>[2x]AEAESALEYAQQALEKAQLALQAARQALKA

In this work, we demonstrate the first ever high-resolution structure of co-assembly between a protein and buckminsterfullerene (C60), which suggests a simple structural mode for protein–fullerene co-organization. As in the protein-only structure, COP forms a canonical tetrameric anti-parallel coiled coil. Each tetramer presents four tyrosine residues (one per monomer) in exterior c positions of the coiled-coil heptad, and each of these engages a C60 moiety. One C60 is wedged between two Tyr residues donated by adjacent tetramers, such that two tetramers are needed to coordinate one C60.

Crystals from the resulting suspension grew within 24 h in several conditions, and three separate structures of the C60Sol–COP complex were resolved to 1.67, 1.76 and 2.35 Å, respectively. Furthermore, the three different COP–C60Sol co-crystals obtained under different conditions all produced effectively identical binding interfaces and assembly geometries, arguing that fullerene may have a strong preference for the observed coordination geometry. The interaction between COP and the fullerene group involves non-polar contacts, with C60 fitting perfectly into a symmetric hydrophobic cavity created by helices of two adjacent COP tetramers. The dominant contact appears to be the π–π aromatic stacking between C60 and Tyr9, donated by each tetramer, while several aliphatic carbons line the pocket to further support the bound pose. The water-solubilizing Tris-acid side chain of C60Sol is not visible in the electron density map. The group likely points into the solvated inner channel of the crystal and is highly mobile as the C60 core rapidly rotates around its centre. On the other hand, there is considerable difference in the arrangement of COP tetramers in the corresponding crystals: COP alone assembles into a body-centered cube, while C60Sol–COP has a honeycomb structure with parallel hexameric channels. In fact, in the fullerene bound structure, no contacts between adjacent COP tetramers occur outside of the C60-binding site. Inter-fullerene nearest-neighbour distances in the C60Sol–COP supercrystal alternate between 1.2 and 1.7 nm. On the other hand, C60Sol–COP supercrystals (of similar dimension as protein-alone crystals) exhibited high electrical conductance (1.40 × 10−7 S, corresponding to resistance of 7.14 × 106 Ω) with at least four orders of magnitude higher currents than in any of the controls.(3~{a}~{S},4~{S},6~{a}~{R})-4,5,6,6~{a}-tetrahydro-3~{a}~{H}-pyrrolo[3,4-d][1,2]oxazole-3,4-dicarboxylic 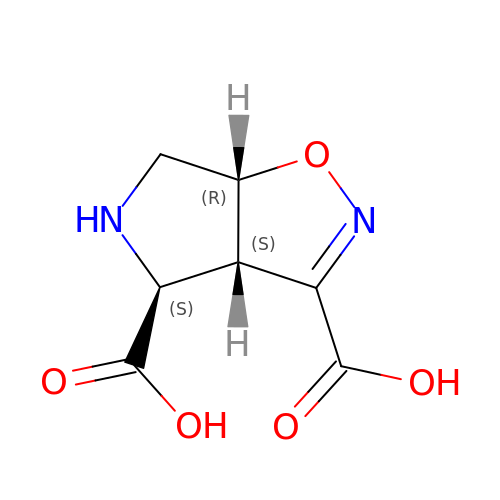acid | C7 H8 N2 O5 | JMTZNIDIUDLCMK-HZLVTQRSSA-N>[2x]GSMDPAIYFKEQFLDGDAWTNRWVES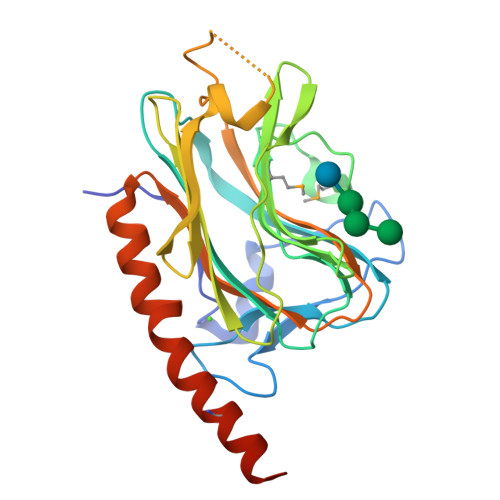KHKSDFGKFVLSSGKFYGDLEKDKGLQTSQDARFYALSAKFEPFSNKGQTLVVQFTVKHEQNIDCGGGYVKLFPSGLDQKDMHGDSEYNIMFGPDICGPGTKKVHVIFNYKGKNVLINKDIRSKDDEFTHLYTLIVRPDNTYEVKIDNSQVESGSLEDDWDFLPPKGSGSGPDANIYAYDSFAVLGLDLWQVKSGTIFDNFLITNDEAYAEEFGNETWGVTKAAEKQMKDKQDEEQRLKLEHHHHHH> MLEEQLYLLACIFASRADTRNIKKLSTRLGSQSKYLEILCVLWPELDDPKNLLFLRELEEEVQSPEGEETTDEDVIVELLESDSSLIPLIESDTTTRSNRYHELQEFISKKLNNKTLENFEEWLRERILICNEMIPETPLLYSVLWETAKSKVLSTKFIGWVEGVLKPLDHLNKRLHLIFKINEWEKMPDSELFKIIFDGVEDMQGYIGIADVIEDELAPTLSYGKKWETFITEFFNKQQFSLKSDTNYQLFIKLYYSLEKGVKDNSEASRKLQSNVVDILFHNSENLFNLSSLTHKLDELWSILSGFPDEITIEEQKTITALE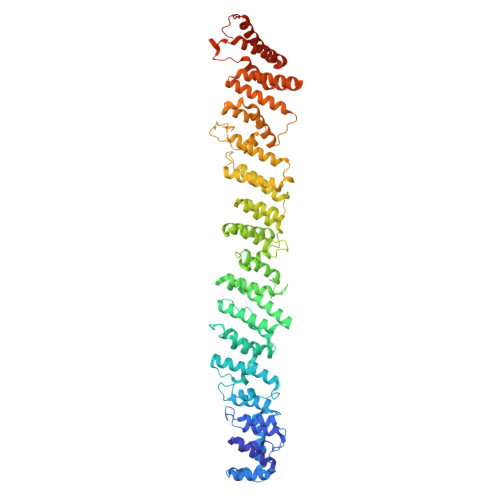MKQFMEFFIKCSTKFSFKEIFAITQEEESAQLAHFSSLCHEEFNKANEISSFLQAMYETVLDISKDDKIFTRISMDEKLYSILEILLQMNEFAYIEAIIERFDYSNNTQIYELLVKFFWHFFNNASNGLRKEPEMKKASQTLQIIQKHMSQRAGTNLTKLEVLLEISDKLSHYSINLNKSHNGARDTAFKPSNILEYRDCPLDIISNLLELNPRLYKDLPTTKSLLFGIYDSLSINREGQTGKVEVDLMVLHIDYALVNLDFGTAYELGKQVFEICQEAGQHMMKALGDEHWLTFYQMGKFVDPNWVDNEIPTEIIVLQMSILGRLLEVCPLEEVEIVTSQWSTLELELSARDLVKDKYALDGQNDNKSKVGGIAREIFHNVTNF>MAAYTLPQLPYAYDALEPHIDARTMEIHHTKHHQTYVDNANKALEGTEFADLPVEQLIQQLDRVPADKKGALRNNAGGHANHSMFWQIMGQGQGQNGANQPSGELLDAINSAFGSFDAFKQKFEDAAKTRFGSGWAWLVVKDGKLDVVSTANQD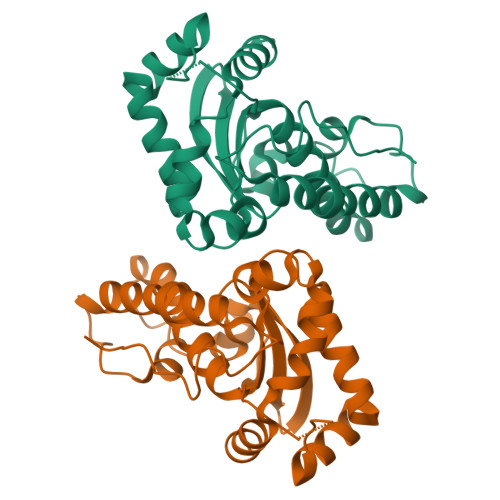NPLMGEAIAGVSGTPILGVDVWEHAYYLNYQNRRPDYLAAFWNVVNWDEVSKRYAAAKLVPRGSAAALEHHHHHH[2x]> NGYEN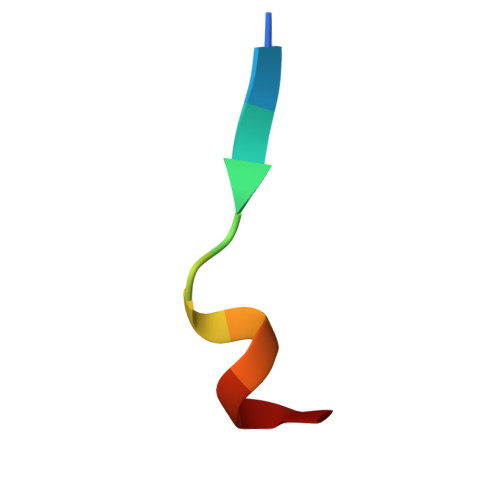PTYKFFE>MSQLQHNIGLSIFEPVAKHRANRIICTIGPSTQSVEALKGLMKSGMSVARMNFSHGSYEYHQTTINNVRAAAAELGLHIGIALDTKGPEIRTGLFKDGEATYAPGDTVLVTTDPAFEKIGTKEKFYVDYPQLPNVVRPGGLIYVDDGVLTLRVLSKEDDCTLKCHVNNHHRLTDRKGINLPGCEVDLPAVSEKDRKDLQFGVEQGVDMIFASFIRTADQVREVRAALGEKGKDTLIISKIE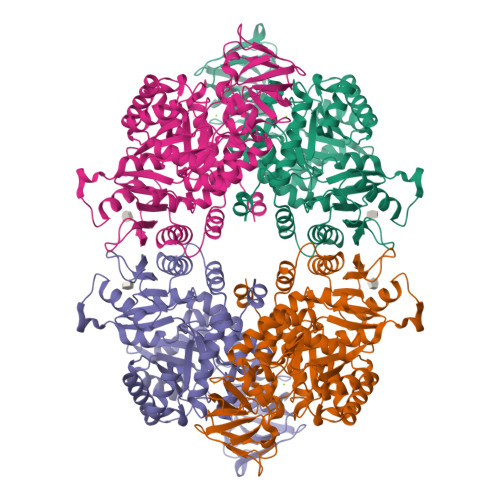NHQGVQNIDAIIEASDGIMVARGDLGVEIPAEKVVVAQMCIISKCNVAGKPVICATQMLESMTTNPRPTRAEVTDVANAVFNGADCVMLSGETAKGKYPNEVVQYMVRICIEAQSATHDSVMFNSIKNLQKIPMSPEEAVCSSAVSSAFEVQAKAILVLSNTGRSARLISKYRPNCPIICATTRLLTCRQLNVTRSVESVYYDVDAHGEDNDREKRVQLGVDWAKTKGYVSAGDVMVIVHADHSVKGYPNQTRLVRVRENLYFQSGGHHHHHH[4x]>[2x]MGSDKIGSHHHHHHENLYFQGMRPIHIAQLDKARPVLILTREVVRPHLTNVTVAPITT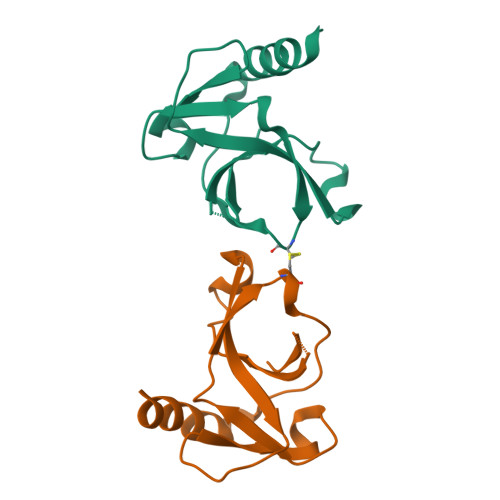TVRGLATEVPVDAVNGLNQPSVVSCDNTQTIPVCDLGRQIGYLLASQEPALAEAIGNAFDLDWVVA> DPTWVDMEAGDIALVKSSWAQIHDKEVDILYNFFKSYPASQAKFSAFAGKDLESLKDTAPFALHATRIVSVINEAIALMGVAENRPALKNVLKQQGINHKGRGVTAAHFEEFETALEAF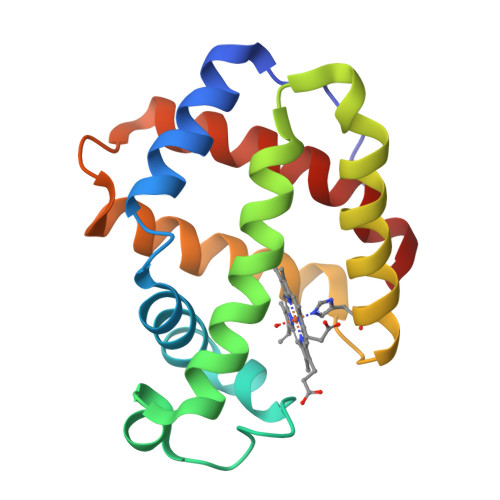LESHASGYNAGTKKAWDSAFNNMYSVVFPEL>GPGMIALEMRNLGGGEILHACPQESLDKPLPCIVFYHGFTSSKLVYSYFAVALAEAGFRVIMPDAPEHGARYQGDEAGRMQRFWPILQQNFREFPALREAIIAEGWLEGERLAVAGASMGGMTALGIMTHHPELNSVACLMGSGYFRSLSQTLFPSPDFDVDSLNEWDVSHQLASLARRPLLLWHGDADDVVPPEETFRLEQALRQGDLAARLTCVWQKGVRHRITPEALA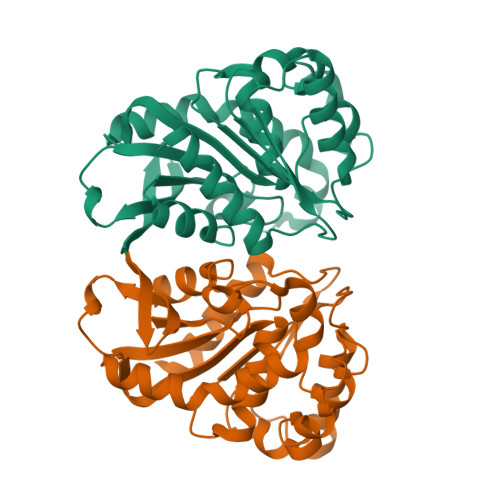TTVAFFQQHLA[2x]> TPTTFVHLFEWNWQDVAQECEQYLGPKGYAAVQVSPPNEHITGSQWWTRYQPVSYELQSRGGNRAQFIDMVNRCSAAGVDIYVDTLINHMAAGSGTGTAGNSFGNKSFPIYSPQDFHESCTINNSDYGNDRYRVQNCELVGLADLDTASNYVQNTIAAYINDLQAIGVKGFRFDASKHVAASDIQSLMAKVNGSPVVFQEVIDQGGEAVGASEYLSTGLVTEFKYSTELGNTFRNGSLAWLSNFGEGWGFMPSSSAVVFVDNHDNQRGHGGAGNVITFEDGRLYDLANVFMLAYPYGYPQVMSSYDFHGDTDAGGPNVPVHNNGNLECFASNWKCEHRWSYIAGGVDFRN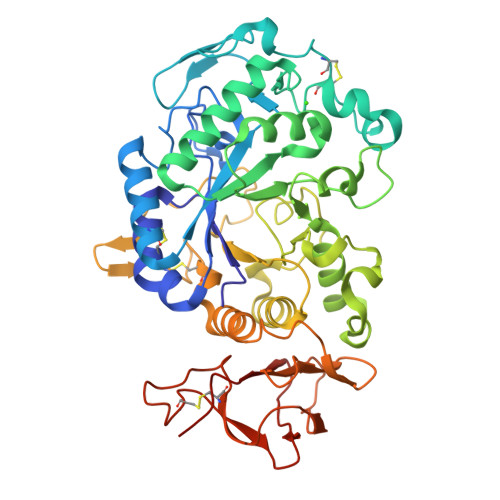NTADNWAVTNWWDNTNNQISFGRGSSGHMAINKEDSTLTATVQTDMASGQYCNVLKGELSADAKSCSGEVITVNSDGTINLNIGAWDAMAIHKNAKLNTSSAS>[2x]MQKIPVKVVTWDEIVSLSTKLAEKIKADEYNVNVIVAIARGG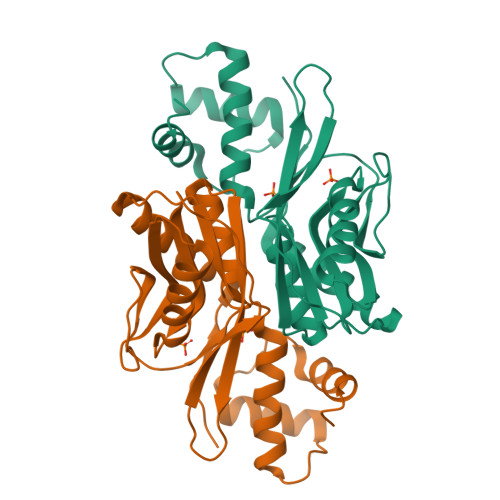LVPARLVADVLGVFDILSIKIEHWIETASHTPEAKVKYPFKVDLSDKNVLIIDDITDTGDSIELARKYVMENFRPTEVKTATLQYIKPAAKIIPDYYAEEIVSWAWFMYPWNYWEDEINLVNKILIERKTKDIDINELKRNFVESYGIENPPISLDKILTEMKRRKIV> MAKGVKKLPKRKGTNPIPRDKWNSDDIARRQLEQDQKLHL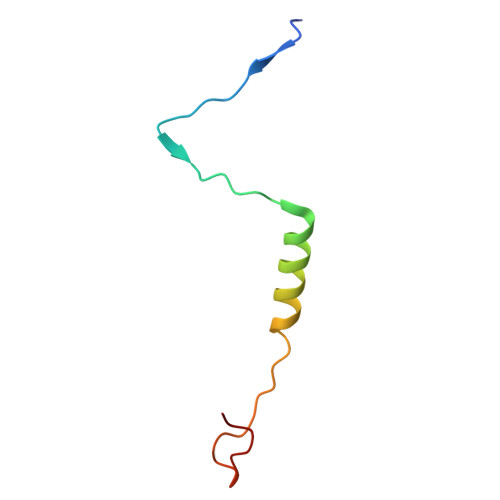TTKGPHTGTNDSFK>[2x]MHHHHHHAAAMETQAGNATGAIKNASDINTGIANLKYDSRDILAVNGDKVESFIPKESINSNGKFVVVEREKKSLTTSPVDILIIDSVVNRTYPGAVQLANKAFADNQPSLLVAKRKPLNISIDLPGMRKENTITVQNPTYGNVAGAVDDLVSTWNEKYSTTHTLPARMQYTESMVYSKSQIASALNVNAKYLDNSLNIDFNAVANGEKKVMVAAYKQIFYT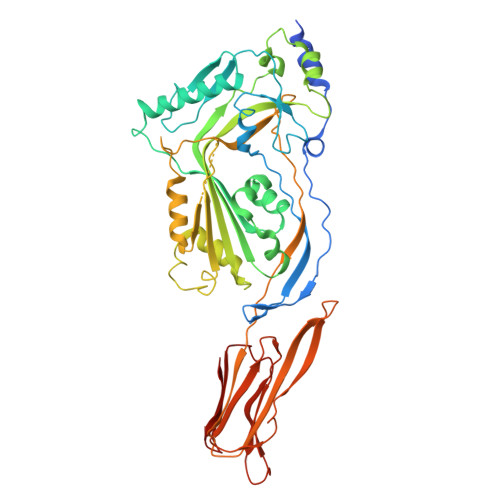VSAELPNNPSDLFDNSVTFDELTRKGVSNSAPPVMVSNVAYGRTVYVKLETTSKSKDVQAAFKALLKNNSVETSGQYKDIFEESTFTAVVLGGDAKEHNKVVTKDFNEIRNIIKDNAELSFKNPAYPISYTSTFLKDNATAAVHNNTDYIETTTTEYSSAKMTLDHYGAYVAQFDVSWDEFTFDQNGKEVLTHKTWEGSGKDKTAHYSTVIPLPPNSKNIKIVARECTGLAWEWWRTIINEQNVPLTNEIKVSIGGTTLYPTATISH>[4x]MKHQHQHQHQHQHQQPLNEEFRPEMLQGKKVIVTGASKGIGREMAYHLAKMGAHVVVTARSKETLQKVVSHCLELGAASAHYIAGTMEDMTFAEQFVAQAGKLMGGLDMLILNHITNTSLNLFHDDIHHVRKSMEVNFLSYVVLTVAALPMLKQSNGSIVVVSSLAGKVAYPMVAAYSASKFALDGFFSSIRKEYSVSRVNVSITLCVLGLIDTETAMKAVSGIVHM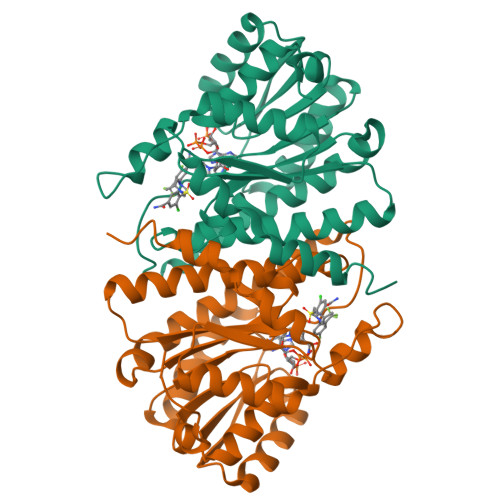QAAPKEECALEIIKGGALRQEEVYYDSSLWTTLLIRNPSRKILEFLYSTSYNMDRFINK>[3x]MVDWELMKKIIESPGVSGYEHLGIRDLVVDILKDVADEVKIDKLGNVIAHFKGSAPKVMVAAHMDKIGLMVNHIDKDGYLRVVPIGGVLPETLIAQKIRFFTEKGERYGVVGVLPPHLRREAKDQGGKIDWDSIIVDVGASSREEAEEMGFRIGTIGEFAPNFTRLSEHRFATPYLDDRICLYAMIEAARQLGEHEADIYIVASVQEEIGLRGARVASFAIDPEVGIAMDVTFAKQPNDKGKIVPELGKGPVMDVGPNINPKLRQFADEVAKKYEIPLQVEPSPRPTGTDANVMQINREGVATAVLSIPIRYMHSQVELADARDVDNTIKLAKALLEELKPMDFTP

Among self-compartmentalized proteases, a new class of dinuclear metalloaminopeptidases complex was recently discovered and named TET due to its tetrahedral shape. TETs are dodecameric particles of 500 kDa and they were first discovered in archaea and then identified in bacteria and eukaryotes. TET1 is a glutamyl-aminopeptidase, TET2 has a broad specificity against neutral amino acids and TET3 shows a preference for positively charged residues such as lysine and arginine. TETs monomers are all formed by a proteolytic domain and a PDZ-like oligomerization domain.

To unambiguously characterize PfTET3, we determined its crystal structure by SAD at 2.5 Å resolution. Purified PfTET3 was crystallized in HEPES 0.1M pH 7.7, NH4CH3COO 0.2 M, 2 mM CoCl2, MPD 44% and Gd-DO3A20 using hanging drop vapor diffusion method. PfTET3Gd crystal was collected at Gd LIII absorption edge. A strong anomalous signal relative to the Gd atoms extends up to 3.0 Å, allowing determining the Gd substructures. The asymmetric unit contains three monomers forming one apex of the PfTET3 tetrahedron. By applying the crystal symmetry operators, PfTET3 dodecamer is reconstituted. M1 is coordinated by residues His314, Asp177, Glu208 and two water molecules, while M2 is coordinated by Asp177, Asp230, His63 and a chloride ion. Indeed, M1 displays an octahedral coordination, while M2 displays a trigonal bypiramidal coordination. By looking to the preferred coordination number of Co2+ and Zn2+, it appears that Co2+ adopts preferentially an octahedral geometry (coordination number of 6), while Zn2+ is often found in a tetrahedral coordination (coordination number 4). These data suggest that M1 is occupied by Co2+ while M2 is occupied by Zn2+. In PfTET3Gd structure, Cl− ion is in the coordination sphere of M2, indicating that M2 is the catalytic metal.> AECSVDIQGNDQFQFNTNAITVDKSCKQFTVNLSHPGNLPKNVMGHNWVLSTAADMQGVVTDGMASGLDKDYLKPDDSRVIAHTKLIGSGEKDSVTFDVSKLKEGEQYMFFCTFPFH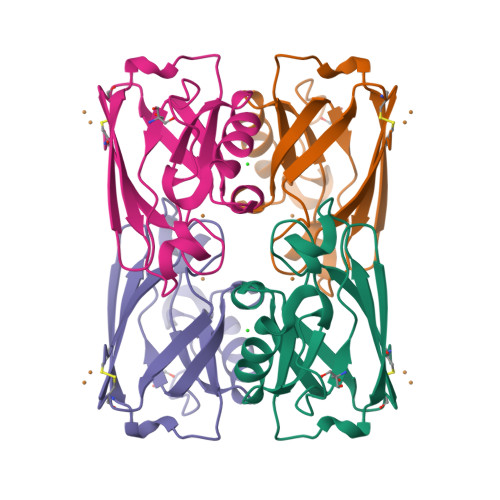SALMKGTLTLK PII proteins are key sensors for the metabolic nitrogen status. Af-GlnK3 shares the canonical fold of PII proteins, consisting of a four-stranded, antiparallel beta sheet and two connecting alpha helices. It forms a tightly packed trimer with approximate dimensions of 30×54 Å. GlnK proteins, when activated, are sequestered to the cytoplasmic membrane where they bind directly to their corresponding Amt proteins, physically blocking ammonium uptake by inserting the T-loops deeply into the transporters' substrate channels.

Af-GlnK3 was isolated without the addition of nucleotides during protein purification, resulting in a structure without any bound ligand and T-loops that were disordered in the crystal packing. Without bound ligands, the T-loops were not found to be fixed in a distinct conformation and were consequently disordered in the crystal structure. Given that the intracellular concentrations of the nucleotide ligands as well as of free Mg2+ are estimated to be rather high, it remains doubtful whether this ligand-free structure is of physiological relevance.

>MKMVVAVIRPEKLECVKKALEERGFVGMTVTEVKGRGEQKGIRLQFRGREVEVDLLQKTKVEVVVSDDAVDEVVEAIVSSARTGKFGDGRIFVIPVEKSVKIRTGDEEVAAAHHHHHH[6x]> FQSNAMKHCPITYEKISDQENYSQRGLHLLSPQ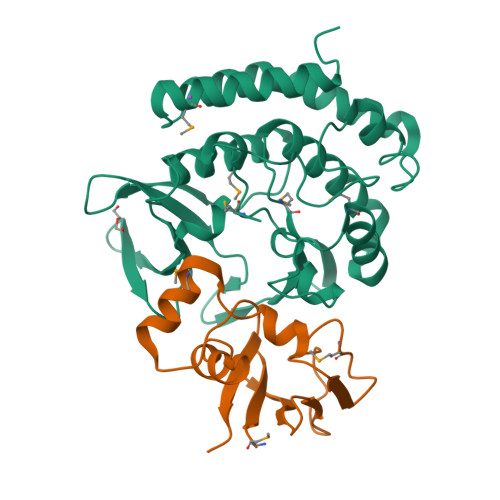LKNLSPLDLSADEQRQEAIARVGKMSVQGVQKKLSAKLKIKEGCFEIVDQYGQYILKPQSDIYPELPENEAITMTLAKTIGLEVPVHGLVYSKDNSLTYFIKRFDRIGHNKKLALEDFAQLSGEDRHTKYKSSMEKVIAVIEQFCTFPKIEFVKLFKLTLFNFLVGNEDMHLKNFSLITKDRKISISPAYDLLNSTIAQKNTKEELALPLKGKKNNLTKSDFLKYFAIEKLGLNQNVIDGIVQEFHQVIPKWQELIGFSFLSQEMQEKYLELLEQRCKRLNFFD;> MRKAYVSVSGIKAGILEELQGGTYQFTYFEDYHGAPVSLTMPLKNKVYDFDVFPPFFEGLLPEGIMLEALLRKYKIDKNDYFGQLILVGQDVVGAVTIEEIR>[2x]EEEELEELAKELEKILRDEEGHLRKLKEALAEGLGDAEEAAELFRAESIDEMKHAEELAKLLKKGGLDPELRELLEELAELELVAINQYREAAEAAAEAAENGSEEARAAAREALEEALALELDGAKLARAALEAVEKLL

The binding and catalytic functions of proteins are generally mediated by a small number of functional residues held in place by the overall protein structure. We describe deep learning approaches for scaffolding such functional sites without needing to pre-specify the fold or secondary structure of the scaffold. We use the methods to design candidate immunogens, receptor traps, metalloproteins, enzymes, and protein-binding proteins, and validate the designs using a combination of in silico and experimental tests. Unlike classical protein design pipelines, which treat backbone generation and sequence design as two separate problems, our methods simultaneously generate both sequence and structure, taking advantage of the ability of RosettaFold to reason over and jointly optimize both data types.

In the training of recent versions of RosettaFold, a subset of positions in the input multiple sequence alignment (MSA) are masked and the network is trained to recover this missing sequence information in addition to predicting structure. This ability to recover both sequence and structural information provides a second solution to the functional site scaffolding problem: given a functional site description, a forward pass through the network can be used to complete, or “inpaint”, both protein sequence and structure in a missing/masked region of protein. Di-iron sites are important in biological systems for iron storage and can mediate catalysis. We were able to recapitulate the di-iron site from E. coli bacterioferritin, composed of four parallel helical segments, to sub-angstrom AF-RMSD using both inpainting and hallucination (the latter were not tested due to buried polar residues). The designs had diverse helix connectivities and low structural similarity to the parent (TM-score 0.55–0.71 to 1BCF_A). We chose 96 inpainted designs to test experimentally, and found that 76 had soluble expression, at least 8 had a spectroscopic shift indicative of Co2+-binding (a proxy for iron binding), and 3 (dife_inp_1–3) had CD spectra consistent with the designed fold and were stabilized by metal binding. Mutation of the metal binding residues abolished binding, and titration analysis of dife_inp_1 suggested that both metal binding sites were successfully scaffolded.>MSELIRVERETGLLTLRLDRQDKKNALTRAMYSRMAEALLEAQADTAVRVVLITGGDACFTSGNDILDFLEQPPSLRDSPVGRFMSALLEFPKPVIAAVNGP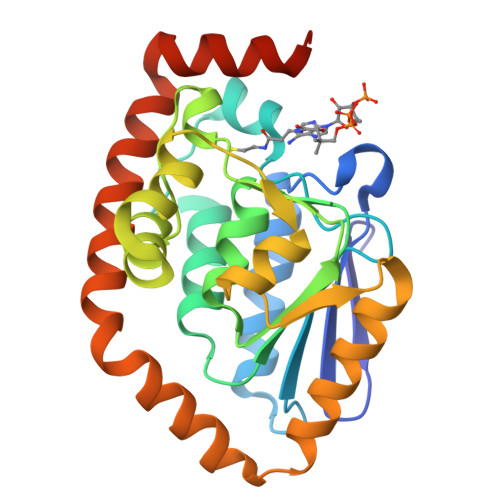AVGIGTTLLLHCDLVFVGRNARLKMPFVNLGLTPEFGSSLILPRMLGHAKAAELLMLGQDFSGEQAAAWGLANAALEDGATVLEHARDAARRFLHLAPSAVVESKRLMKAPFIEELRRVIAEEGDIFSTRLRSPEAIEALSAFMHRRQPDFSRFA[2x]>[2x]MRGSHHHHHHGMASMNRTILVPIDISDSELTQRVISHVEAEAKIDDAKVHFLTVIPSLPYYASLGLAYSAELPAMDDLKAEAKSQLEAII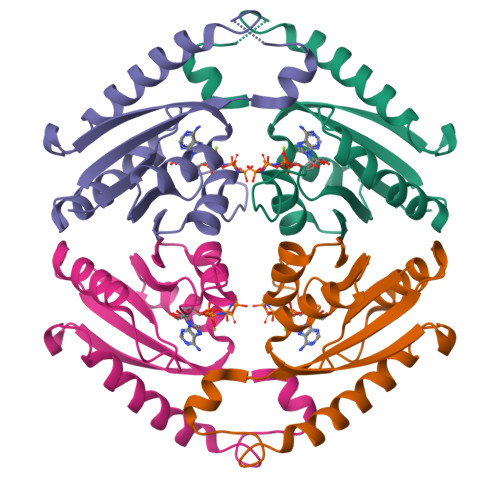KKFNLPADRVQAHVAEGSPKDKILEMAKKLPADMVIIASHRPDITTYLLGSNAAAVVDHAECSVLVVR> GGAACUUAUUCAUUAUACCCCUCAUUUUCGAGUGAGGCGGAUUAGAUUCGUCUGAUCGUAGUGGUGGUGGCUUGCUUCGGCGAGCCCGGCAGGCCUUCGGGCUUGCUCAGGGGUUCGCUCCUGAGAUUAUCAUCCAACCUCCAAGGAUGGUAAUCCGGCGUCGAUUGUAAGGUCUAAACAAUUGACGCACCACUACUACAGUCCCAACGACUGAGGGACUCGUCGACUCGGUUAAGAUCGGAAACCGGGUCGAGGUAUAGUGAAUGAGUUCCAAUUCUCCAUUUACGGCAUCUUGUGCGAACCGAUCACGCACGAGAUGGUCCUUACGGGGUGUCCCAACAGUCGAGGGGCACGCAGGAUGCCUAGAAUAGACCACUAGGUAUCCUCAGUGCGCCAUGCAAUGGAGGAGCAUGGUGCACUGCAGGGCUCCUGAAAAGGAGUCCUGGCAGAAGGGUUCGCCUUUCUCCCGUAGGGACGACU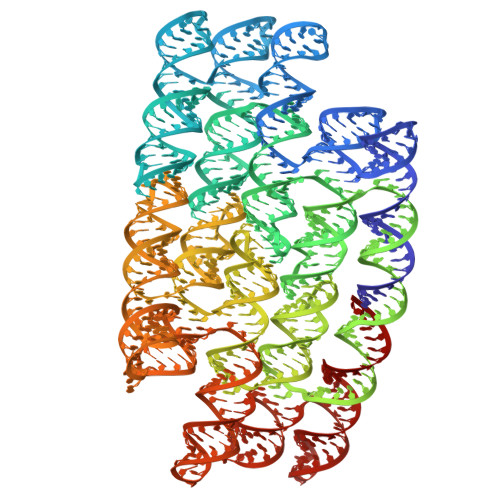UUCUUUGAAAAAAGGAAGUCCCAGUUUGCUUCGGCGAACUCCGACUCUAGGAAACUAGGGUCGGGUAGAUGGAGAAUU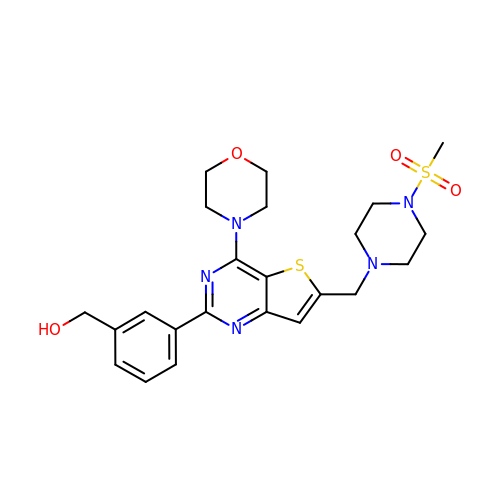[3-(6-{[4-(methylsulfonyl)piperazin-1-yl]methyl}-4-morpholin-4-ylthieno[3,2-d]pyrimidin-2-yl)phenyl]methanol | C23 H29 N5 O4 S2 | UTNWCQOGZIRULH-UHFFFAOYSA-N> HHHHHHGDAPGGAHMTAQTVTGAVAAAQLGATLPHEHVIFGYPGYAGDVTLGPFDHAAALASCTETARALLARGIQTVVDATPNGCGRNPAFLREVSEATGLQILCATGFYYEGGGATTYFKFRASLGDAESEIYEMMRTEVTEGIAGTGIRAGVIKLASSRDAITPYEQLFFRAAARVQRETGVPIITHTQEGQQGPQQAELLTSLGADPARIMIGHMDGNTDPAYHRETLRHGVSIAFDRIGLQGIVGTPTDAERLSVLTTLLGEGYADRLLLSHDSIWHWLGR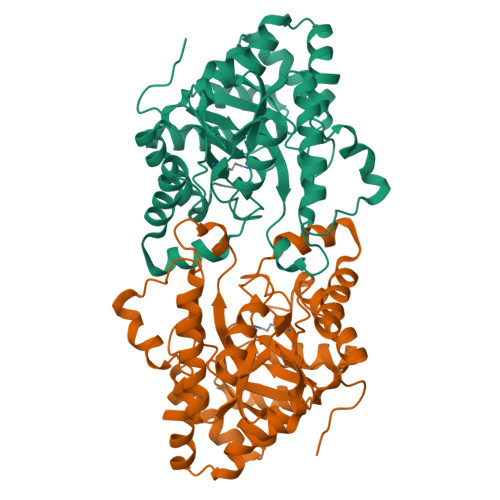PPAIPEAALPAVKDWHPLHISDDILPDLRRRGITEEQVGQMTVGNPARLFG> MSGDSVAPHQRAACEQLHSEYKQCLAKNGRTHFSACTDFHSKLRACENMLGTSYCIDEGINLMKCTKNPDPSFCAKEFVAMRECNRPQGPHLVLSSSPSSPPHYELRPEVKHLYNVDSTDLGSAVAPVRSKEQLDRVADSLKADLNLPGYGHIPYKWESLRP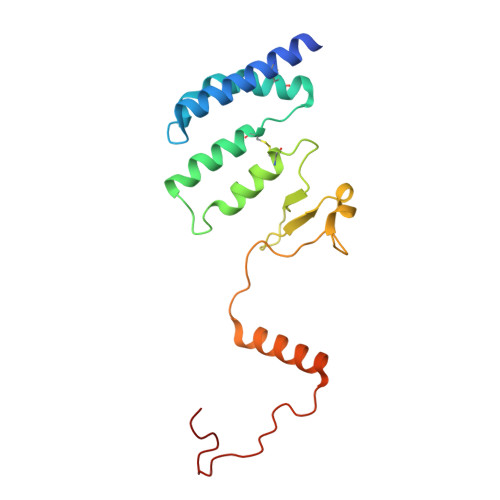NPGA>MTNLQTFLDIATEAALAAGAVLQGYLGKLEDAITEKGRPGDLVTAADKASEAVVLEIIRRHFPQHSILAEESGKLGNQDNEYLWAIDPLDGTTNYAHQYPAFCVSIGLLINGVPQVGVIYDPFHDELFRGAAGLGATRNRRPIKVSDTSELS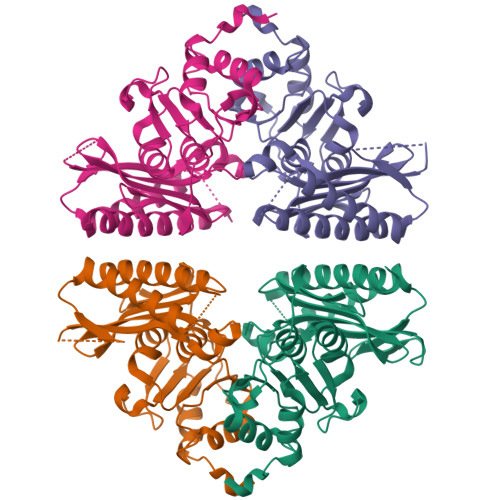KSLLVTGFAYDRRETPDNNYAEFCHLTHLTQGVRRSGSAALDLAHVACGRVDGYWERGISPWDVVAGVILLEEAGGKVTAYDSTPLKIATGRILATNGSIHDNLSRALMQVPPLSAWE[4x]>LPRETDEEPEEPGKKGSFVEMVDNLRGKSGQGYYVEMTVGSPPQTLNILVDTGSSNFAVGAAPHPFLHRYYQRQLSSTYRDLRKGVYVPYTQGKWEGELGTDLVSIPHGPNVTVRANIAAITESDKFFINGSNWEGILGLAYAEIARPDDSLEPFFDSLVKQTHVPNLFSLQLCGAGFPLNQSEVLASVGGSMIIGGIDHSLYTGSLWYTPIRREWYYEVIIVRVEINGQDLKMDCKEYNYDKSIVDSGTTNLRLPKK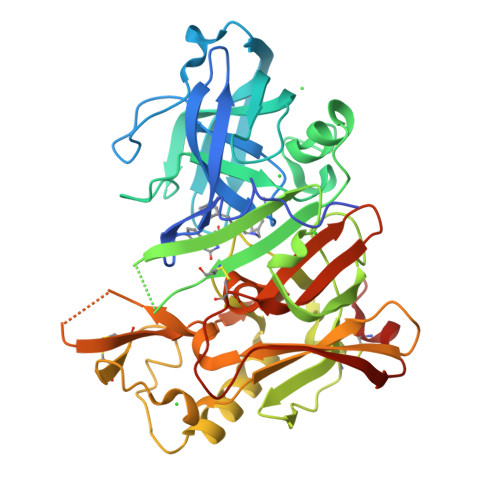VFEAAVKSIKAASSTEKFPDGFWLGEQLVCWQAGTTPWNIFPVISLYLMGEVTNQSFRITILPQQYLRPVEDVATSQDDCYKFAISQSSTGTVMGAVIMEGFYVVFDRARKRIGFAVSACHVHDEFRTAAVEGPFVTLDMEDCGYNIPQTDEST[3x]5-(5-aminopent-1-yn-1-yl)-2'-deoxycytidine 5'-(tetrahydrogen triphosphate) | C14 H25 N4 O13 P3 | 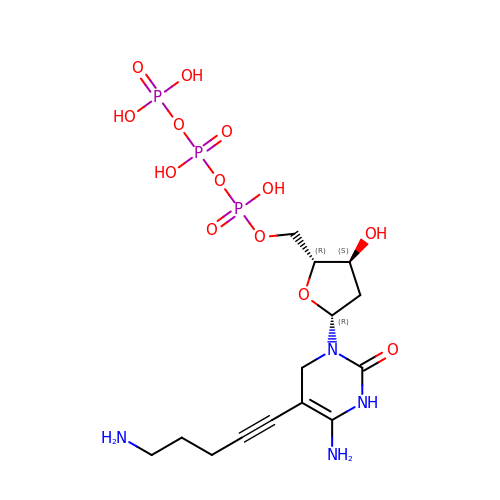QDKMIMUSGQEUSC-QJPTWQEYSA-N>MRAKTKLIHGIRIGEPSTGSVNVPIYQTSTYKQEAVGKHQGYEYSRTGNPTRAALEEMIAVLENGHAGFAFGSGMAAITATIMLFSKGDHVILTDDVYGGTYRVITKVLNRFGIEHTFVDTTNLEEVEEA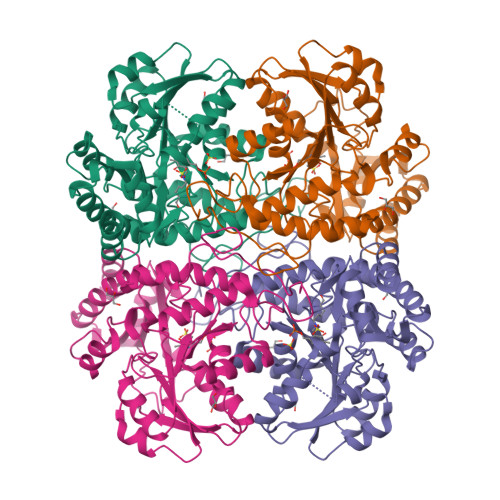IRPNTKAIYVETPTNPLLKITDIKKISTLAKEKDLLTIIDNTFMTPYWQSPISLGADIVLHSATKYLGGHSDVVAGLVVVNSPQLAEDLHFVQNSTGGILGPQDSFLLLRGLKTLGIRMEEHETNSRAIAEFLNNHPKVNKVYYPGLESHQNHELATEQANGFGAIISFDVDSEETLNKVLEKLQYFTLAESLGAVESLISIPSQMTHASIPADRRKELGITDTLIRISVGIEDGEDLIEDLAQALA[2x]> QPIFLNVLEAIEPGVVCAGHDNNQPDSFAALLS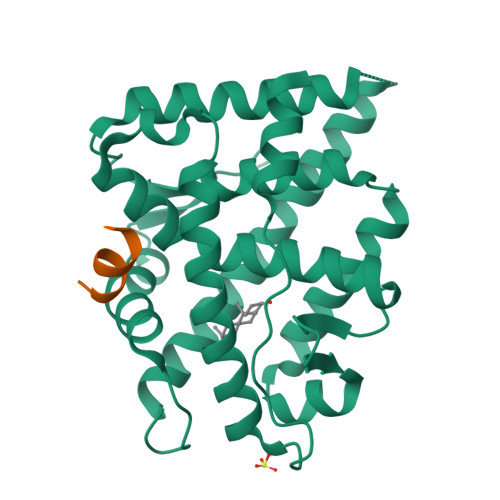SLNELGERQLVHVVKWAKALPGFRNLHVDDQMAVIQYSWMGLMVFAMGWRSFTNVNSAMLYFAPDLVFNEYRMHKSRMYSQCVRMRHLSQEFGWLQITPQEFLCMKALLLFSIIPVDGLKNQKFFDELRMNYIKELDRIIACKRKNPTSCSRRFYQLTKLLDSVQPIARELHQFTFDLLIKSHMVSVDFPEMMAEIISVQVPKILSGKVKPIYFHTQ;> RGAFQNLFQSV>[3x]AATAPAGASTTSSTSSAQKSFFKTTEMIGYVHSIDGTIATLIPAPGNPGVAYNTIIQIQVSPTTFAAGLVFNLEKDGRIGIILMDNITEVQSGQKVMATGQLLHIPVGAGVLGKVVNPLGHEVPVGLVTRSRRLLDSTLGKVDTGAPNIVSRSPVNYNLLTGFKAVDTMIPIGR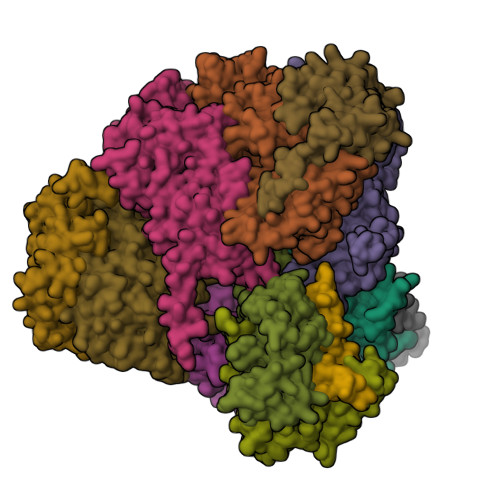GQRELIVGDRQTGKTSIAVSTIINQVRINQQILSKNAVISIYVSIGQRCSNVARIHRLLQSYGALRYTTVMAATAAEPAGLQYLAPYAGVTMGEYFMNRGRHCLCVYDDLSKQAVAYRQISLLLRRPPGREAYPGDVFYLHSRLLERAAMLSPGKGGGSVTALPIVETLSNDVTAYIVTNVISITDGQIYLDTKLFTGGQRPAVNIGLSVSRVGSSAQNAAMKGVAGKLKGILAEYRKLAADSVGGQQVQTIPMIRGARFVALFNQKQPSYFMNAIVSLYACLNGYLDDVKVQYVKFYEYLLVHRDLGIMYGTAKNKFFYMYVQELNYLIRFFTLNSPILHGELEEMLKQHTHLFLQHYQSKMNAIKSEKDVKALKNLLYSCKRAV;>ASTAPVADHKGRVGHVSQVIGAVVDVHFADGVPPVLTALDVVDKLGRDEPLTLEIVQHLDAHTGRCIAMQTTDLLKLKAKVVSTGGNISVPVGRETLGRIFNVLGDAIDQRGPVGEKLRMPIHAVAPKLADQAAEDAVLTTGIKVIDLILPYCKGGKIGLFGGAGVGKTVIIMELINNVAKGHGGFSVFAGVGERTREGTDLYLEMMQSKVIDLKGESKCVLVYGQMNEPPGARARVAQSALTMAEYFRDVEGQDVLLFIDNIFRFTQANSEVSALLGRIPAAVGYQPTLAEDLGQLQERITSTTKGSITSVQAVYVPADDITDPAPATTFSHLDATTVLDRAVAESGIYPAVNPLECASRIMDPDVISVDHYNVAQDVVQMLTKYRELQDIIAVLGIDELSEEDKLIVDRARKLVKFLSQPFQVAEVFTGMTGHYVQLDDTIDSFSGLLMGTYDQVPEMAFYMVGGINSVLEKAKKMAEEAAELEKMRRARVAQASS[3x];> SGKLRLYKEKLEGYNRFYSIVKTIKMVTLAKYRAAQGRIRTRDFSLRYTELAFSKPQASRDAVAAAKNALVYIPITTNRGSCGALNSNIVRCIDSVVSSKMVLMPVGKRGIDSFSKLYPDEFRYGIINDMKESMHFGYATFVIENAYEVSKDADRYQVIFNRFVSAGVQRNAVYNIPSYEKWKEDLADAASSDNQKNRYLFANALQNEEEQLIRDFFDFHAALAVLNAVGENELSEQAARLVAVEGQLTNISSLQQRTSSLYNKTRQFGITAALIEILSAMSSLEGNAMKGVRRNKFWEGAVTK;> QSAPHDLPEGFEFMEHKVVNKDIHAPHENLETLRLTLTRQDEFLLREEPVKCVTVTGTNGEYGIYPGHAYKIVQLNPSPLTVEYTDGTTKKYFVSGGFAHINNEGSCDVNTVECTLLDDLDLAIAEKELAAQQAALGSAKDDKAKSVVEIRISVIEAVIAALKHH;> SSSWRDHGISYLKYLNVCTETLHSTVKESRRAKYERWSKPCYTAQRPDGAGGQETIDKVPIHTKDY;>AATSAAKKYDLFGYEVDTNTAPWIEKIKKCKYYDEAGEVLVNMNVSNCPPDIATYNATLQCIYQSPSKQSTPVDNESKFCAMMDLLEEMQHRNRLKPNEESWTWVMKECVKSGQFRLGYCIQQVMETECKGCPADLVKANEANAQKAKTEGKEHPGHLSQQAGLFDVKVE[3x]(1H-1,2,3-triazol-1-yl){4-[4-(trifluoromethyl)phenyl]piperazin-1-yl}methanone 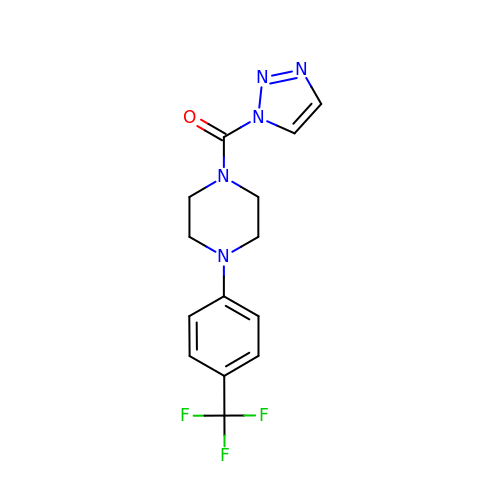| C14 H14 F3 N5 O | HHQYTTYRIFYYCO-UHFFFAOYSA-N Cysteine tryptophylquinone (CTQ) is a protein-derived quinone cofactor initially identified in quinohemoprotein amine dehydrogenase (QHNDH), a bacterial enzyme that catalyzes oxidative deamination of various aliphatic primary amines for use as energy, carbon, and nitrogen sources. Here, we shed light on the qhpG gene, which has been predicted to encode a flavoprotein monooxygenase, directly involved in CTQ biogenesis. Biochemical evidence reported herein proves that QhpG is an atypical single-component monooxygenase, catalyzing dihydroxylation of an unmodified Trp residue in the protein substrate. Based on these results, we concluded that the CTQ-precursor Trp43 is doubly hydroxylated, most likely at 6- and 7-positions of the indole ring, by the QhpG reaction.

In the crystal, each asymmetric unit contained two monomers that are related by a non-crystallographic (NCS) two-fold axis and packed compactly. Thus, the dimerization is assumed to be a crystallographic artifact. Each monomer consists of a large N-terminal catalytic domain (residues 1–344) and a small C-terminal winged-helix (WH) domain (residues 349–429), with a large pocket between the two domains. The catalytic domain of QhpG contains a glutathione reductase-type Rossmann-fold for FAD binding, in which FAD is bound between two lobes of the catalytic domain, showing a clear Fo–Fc omit map for the entire FAD molecule. Briefly, the isoalloxazine ring of FAD is sandwiched by the side chains of Pro267 and Glu42/Arg240 from the re- and si-faces, respectively. The di-phosphate moiety interacts with the side chains of Arg36 and Arg89, and the main chain NH groups of Ala14 and Asp260. Two channels connecting the molecular surfaces to the re- and si-faces of the isoalloxazine ring of FAD have been identified. The narrow and deep re-face channel is open at the bottom of the large pocket between the two domains and composed of the main chains of Gly43–Val44 and Ser269–Asn271, and several hydrophobic residues (Val72, Trp74, Val174, Trp181, Trp183, Leu268, and Phe322), most of which are conserved in SvCmlS and QhpG orthologs. The side chains of Glu42 and Arg240 are apart by ~4.5 Å from each other, suggesting a weak electrostatic interaction, and are located over the middle of the isoalloxazine ring. It is possible that Glu42 and Arg240 act as a lid for the si-face channel, through which dissolved dioxygen is able to access to the isoalloxazine ring.

>GHMAEPRIVVLGAGPAGAATAIGLRRLGYAVTVVSEWRRFAAVEGVSQRVLEGLRHVGLGGALRQAAMPATRQVHWNGQQLHLNQEFLLDRQRFDRALRDDLQRAGVSVVEGRVREVVRDVGHGIRLDDGQVLQADFLVEARGRQAPLAADRLRGPETVSLLNVWQAAPGAPASAVESLADGWAWMARLEDGRCYWQVTLDAAGLPGKAGLADYCAARRADSALVTELFDARALASAEVHARSSTAILAGECVGQDWIRVGDAAMAVDPLSGNGIFQSLSSALQAPVVINTLLRRPERAGLARQFHQQRIEQLFLRFARIGRDFYGQEQGRVGQPFWARRQGWPDMQALHVAADWSAVRVERRPVLRDGLVDEAEVVVTADQPLGVWHLQGVELAPAVRELQAGRPLEAVVSGLSGEQQRMVRRWLLEQGLV[2x]ROXITHROMYCIN 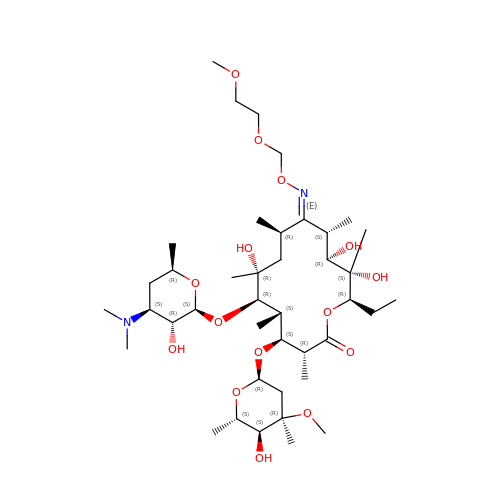| C41 H76 N2 O15 | RXZBMPWDPOLZGW-XMRMVWPWSA-N Mechanosensitive channels respond to mechanical forces exerted on the cell membrane and play vital roles in regulating the chemical equilibrium within cells and their environment. The MscS-like channels are homoheptamers, with each monomer comprising a cytoplasmic domain and a transmembrane (TM) domain. YnaI is paralogous to MscS with a similar architecture. YnaI’s most distinct feature is that its transmembrane domain contains five TMs instead of three for MscS.

Here we report the cryo-EM structures of the SMA2000-purified wild-type YnaI at an overall resolution of 2.4 Å. Consistent with the previously reported structures, 3D reconstruction of YnaI directly extracted from the cell membrane with SMA2000 reveals a heptamer. We could reconstruct the soluble portion for YnaI at high resolution; however, we could only resolve TM5 and TM4 of its transmembrane region. EM density for seven potential lipid molecules was found in the hydrophobic pockets defined by TMs 4–5 and the cytoplasmic region. In the E. coli inner cell membrane, phosphatidylethanolamine (PE) is the predominant lipid species, and this molecule also fits well into those densities. Therefore, we tentatively built PE molecules into the corresponding densities. Overall, YnaI appears in a closed state defined by the minimal diameter of the pore formed by TM5a ~13 Å, similar to the closed state of YnaI in DIBMA (14 Å). The lipid observed is bound in the juxtamembrane area defined by two TM5b helices and a loop from the β-domain, which forms a protein-lipid interface. The negatively charged phosphate head fits well within the positively charged pocket formed by R116, S119, R120, K123, Y174, W201, and R202. In our structure of YnaI solubilized in SMA2000, TM4 (MscS TM2) is shifted by about ~15° or ~2.8 Å compared to the other published structures.

>MIAELFTNNALNLVIIFGSCAALILMSFWFRRGNRKRKGFLFHAVQFLIYTIIISAVGSIINYVIENYKLKFITPGVIDFICTSLIAVILTIKLFLLINQFEKQQIKKGRDITSARIMSRIIKITIIVVLVLLYGEHFGMSLSGLLTFGGIGGLAVGMAGKDILSNFFSGIMLYFDRPFSIGDWIRSPDRNIEGTVAEIGWRITKITTFDNRPLYVPNSLFSSISVENPGRMTNRRITTTIGLRYEDAAKVGVIVEAVREMLKNHPAIDQRQTLLVYFNQFADSSLNIMVYCFTKTTVWAEWLAAQQDVYLKIIDIVQSHGADFAFPSQTLYMDNITPPEQGR[7x]>MRGSHHHHHHGSMTDTYLHETLVFDNKLSYIDNQRDTDGPAILLLPGWCHDHRVYKYLIQELDADFRVIVPNWRGHGLSPSEVPDFGYQEQVKDALEILDQLGVETFLPVSHSHGGWVLVELLEQAGPERAPRGIIMDWLMWAPKPDFAKSLTLLKDPERWREGTHGLFDVWLDGHDEKRVRHHLLEEMADYGYDCWGRSGRVIEDAYGRNGSPMQMMANLTKTRPIRHIFSQPTEPEYEKINSDFAEQHPWFSYAKLGGPTAFPAIDVPDRAAVHIREFATAIRQGQ[2x]

Arthrobacter nitroguajacolicus Rü61a 1-H-3-hydroxy-4-oxoquinaldine 2,4-dioxygenase (HOD) and Pseudomonas putida 33/1 1-H-3-hydroxy-4-oxoquinoline 2,4-dioxygenase (QDO) were the first dioxygenases discovered to belong to the ABH-fold family. They catalyze the O2-dependent breakdown of N-heteroaromatic quinolone-type substrates with concomitant carbon monoxide production. Atypical for oxygenases, these enzymes promote the activation of the triplet ground-state O2 molecule without the aid of metal centers or external organic co-factors. Kinetic measurements indicate that their reaction mechanism relies on a fast initial step, during which the substrates' 3-hydroxyl group is deprotonated by the His-Asp subset of the triad, thus promoting its activation for molecular oxygen attack (step 1), whilst the nucleophile is not essential.

Normoxic and hyperoxic HODH251A–MQO structures validate S101 as an O2/H2O modulator. MQO, a non-reactive molecule structurally closest to the natural substrate, in which the hydroxyl group at position 3 is replaced by the –H substituent. As crystals of HODH251A typically diffract better than those of wild-type HOD we solved the X-ray structure of this variant in complex MQO under normoxic and hyperoxic conditions at the 2.0 Å and 2.1 Å, resolution, respectively (Table S1†). We next inspected electron density maps following the O2-pressurization experiment (40 bar O2 for 2 minutes). These do not reveal changes that we could positively ascribe to O2 bound at the R-site. Instead of the elongated electron-rich density observed for bound dioxygen in other systems, O2-pressurization led to a decrease in electron density at the R-site compared to that under normoxic conditions. Occupancy refinement of a water molecule at this location gives values of 0.67 and 0.48 in the two independent molecules present in the a.u. Remarkably, S101 shifts completely to the trans rotamer (χ1 values of 180.08 and 180.66°) with no indication of the alternative plus rotamer observed under normoxic conditions. Overall, these observations indicate that O2 most likely interferes with H2O binding at the R-site, and although disorder negates its positive identification, this nevertheless leads to the shift of S101 to the trans rotamer that, in agreement with the simulations, appears to be positively correlated with the presence of dioxygen at the R-site.> EVKQENRLLNESESSSQGLLGYYFSDLNFQAPMVVTSSTTGDLSIPSSELENIPSENQYFQSAIWSGFIKVKKSDEYTFATSADNHVTMWVDDQEVINKASNSNKIRLEKGRLYQIKIQYQRENPTEKGLDFKLYWTDSQNKKEVISSDNLQLPELKQKSSNSRKKRSTSAGPTVPDRDNDGIPDSLEVEGYTVDVKNKRTFLSPWISNIHEKKGLTKYKSSPEKWSTASDPYSDFEKVTGRIDKNVSPEARHPLVAAYPIVHVDMENIILSKNEDQSTQNTDSQTRTISKNTSTSRTHTSEPGSNSNSSTVAIDHSLSLAGERTWAETMGLNTADTARLNANIRYVNTGTAPIYNVLPTTSLVLGKNQTLATIKAKENQLSQILAPNNYYPSKNLAPIALNAQDDFSSTPITMNYNQFLELEKTKQLRLDTDQVYGNIATYNFENGRVRVDTGSNWSEVLPQIQETTARIIFNGKDLNLVERRIAAVNPSDPLETTKPDM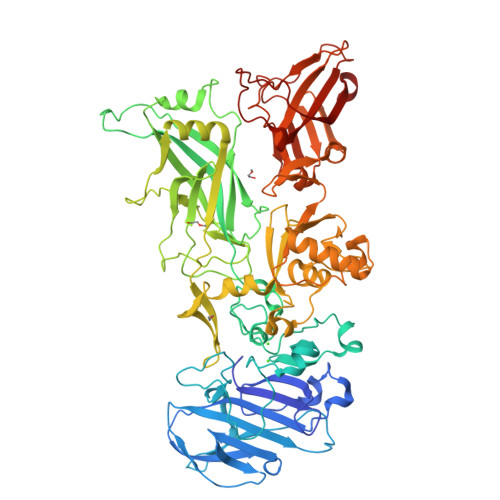TLKEALKIAFGFNEPNGNLQYQGKDITEFDFNFDQQTSQNIKNQLAELNATNIYTVLDKIKLNAKMNILIRDKRFHYDRNNIAVGADESVVKEAHREVINSSTEGLLLNIDKDIRKILSGYIVEIEDTEGLKEVINDRYDMLNISSLRQDGKTFIDFKKYNDKLPLYISNPNYKVNVYAVTKENTIINPSENGDTSTNGIKKILIFSKKGYEIG>[8x]MGSHHHHHHGRSAAGTMANLDKMLNTTVTEVRQFLQVDRVCVFQFEEDYSGVVVVEAVDDRWISILKTQVRDRYFMETRGEEYSHGRYQAIADIYTANLTECYRDLLTQFQVRAILAVPILQGKKLWGLLVAHQLAAPRQWQTWEIDFLKQQAVVVGIAIQQS

By applying 17 rounds of molecular evolution to the GAF domain of PCB-binding NpR3784 CBCR, we have developed the first CBCR-based NIR FP, which efficiently binds endogenous BV and fluoresces in various mammalian cells. With molecular weight of only 17 kDa, miRFP670nano is the smallest monomeric NIR FP that fluoresces in mammalian cells as bright as twice bigger state-of-art two-domain NIR FPs. After each round, we tested the best clones in mammalian cells and selected for the next molecular evolution only those which exhibited the high fluorescence brightness in both bacteria and mammalian cells. Totally, 17 rounds of the directed molecular evolution resulted in an NIR FP variant, termed miRFP670nano, consisting of 147 amino acid residues (17 kDa) and bearing 18 substitutions (numbering follows that for miRFP670nano sequence) relative to wild-type GAF from NpR3784: V7M, F25C, M26V, Y27F, P31E, S41A, A48S, N51K, Q55R, T57R, I72Y, G82N, H87Y, N99I, N117H, C119L, L136Q, and Q139V. miRFP670nano efficiently binds endogenous BV in mammalian cells.

To reveal the structural basis of the protein stability, brightness, and specificity to BV chromophore, we determined the crystal structure of miRFP670nano at 1.95 Å resolution. miRFP670nano adopts a GAF-domain fold, but with the N and C termini located in the spatial proximity. BV is covalently attached by a thioether bond between the conserved for CBCRs Cys86 residue and the C31 atom of the ring A, similar to the native CBCR’s PCB chromophore, but having a double bond between C31 = C32. This mode of the BV binding is different than in natural BphPs and red-shifted BphP-derived NIR FPs in which BV is attached via the C32 atom of the ring A to a conserved Cys in the PAS domain. In the chromophore-binding pocket, BV is stabilized by eight hydrogen bonds with D56, Y67, T84, R71, and H117, π–π stacking with Y87, and T-stacking with F59. Of the 18 amino acid substitutions introduced into parental NpR3784g, F25C, Y27F, H87Y, N99I, and N117H are located within 3.6 Å of the chromophore and either directly stabilize it or provide for it favorable accommodation. One of the important substitutions, N117H makes a strong H-bond with the ring D, which is absent in NpR3784g, thus preventing rotation of this ring and non-radiative energy dissipation via photoswitching. Another critical mutation is H87Y, which introduced a perfect parallel π–π stacking with BV. F25C makes additional space in the chromophore-binding pocket, possibly enhancing BV accommodation. T57R substitution introduced a flexible positively charged residue near the chromophore binding site, enabling electrostatic attraction of BV and its additional shielding from solvent. Substitutions Y27F and N99I increased the hydrophobicity of the chromophore environment.>QQASTLPDLAEQFAPPDVAPPLLIKLVKAIEKKGLECSTLYRTQSSSNPAELRQLLDCDTASLDLEMFDVHVLADAFKRYLLDLPNPVIPVAVSSELISLAPEVQSSEEYIQLLKKLIRSPSIPHQYWLTLQYLLKHFFKLSQTSSKNLLNARVLSELFSPLLFRFPAASSENTEHLI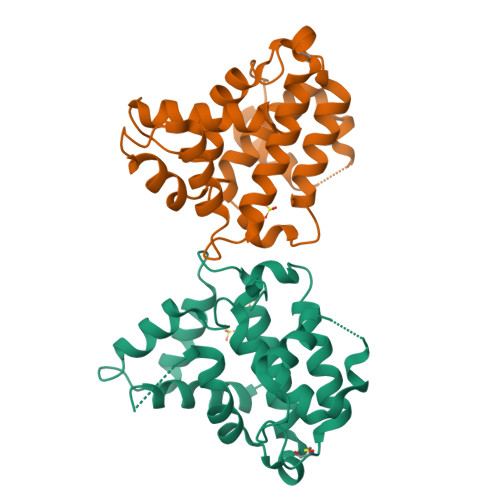KIIEILISTEWNERQ[2x]>GAGSTAGKVIKCKAAVLWEEKKPFSIEEVEVAPPKAHEVRIKMVATGICRSDDHVVSGTLVTPLPVIAGHEAAGIVESIGEGVTTVRPGDKVIPLFTPQCGKCRVCKHPEGNFCLKNDLSMPRGTMQDGTSRFTCRGKPIHHFLGTSTFSQYTVVDEISVAKIDAASPLEKVCLIGCGFSTGYGSAVKVAKVTQGSTCAVFGLGGVGLSVIMGCKAAGAARIIGVDINKDKFAKAKEVGATECVNPQDYKKPIQEVLTEMSNGGVDFSFEVIGRLDTMVTALSCCQEAYGVSVIVGVPPDSQNLSMNPMLLLSG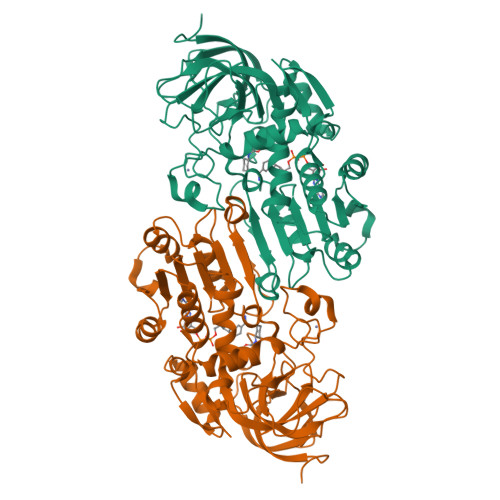RTWKGAIFGGFKSKDSVPKLVADFMAKKFALDPLITHVLPFEKINEGFDLLRSGESIRTILTF[2x]>RNLMIVDGTNLGFRFKHNNSKKPFASSYVSTIQSLAKSYSARTTIVLGDKGKSVFRLEHLPEYKGNRDEKYAQRTEEEKALDEQFFEYLKDAFELCKTTFPTFTIRGVEADDMAAYIVKLIGHLYDHVWLISTDGDWDTLLTDKVSRFSFTTRREYHLRDMYEHHNVDD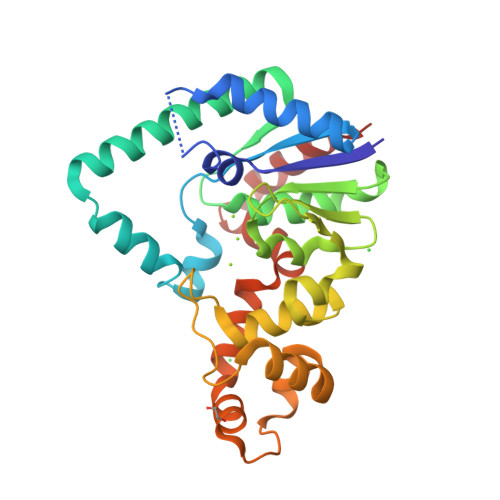VEQFISLKAIMGDLGDNIRGVEGIGAKRGYNIIREFGNVLDIIDQLPLPGKQKYIQNLNASEELLFRNLILVDLPTYCVDAIAAVGQDVLDKFTKDILEIAE[2x]>[4x]MSLVEKQSALESKARSWLIERGVEIDDIAELVLFLQQKYHPGLELDICRQNVEHVLRKREVQNAVLTGIQLDVMAEKGELVQPLQNIISADEGLYGVDEILALSIVNVY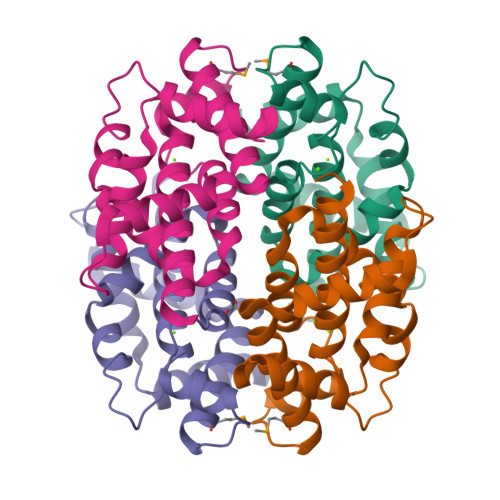GSIGFTNYGYIDKVKPGILAKLNEHDGIAVHTFLDDIVGAIAAAAASRLAHSYHDDIVNEGGSHHHHHH> AMDPEFETGEVVDCHLSDMLQQLHSVNASKPSERGLVRQEEAEDPACIPIFWVSKWVDYSDKYGLGYQLCDNSVGVLFNDSTRLILYNDGDSLQYIERDGTESYLTVSSHPNSLMKKITLLKYFRNYMSEHLLKAGANITPREGDELARLPYLRTWFRTRSAIILHLSNGSVQINFF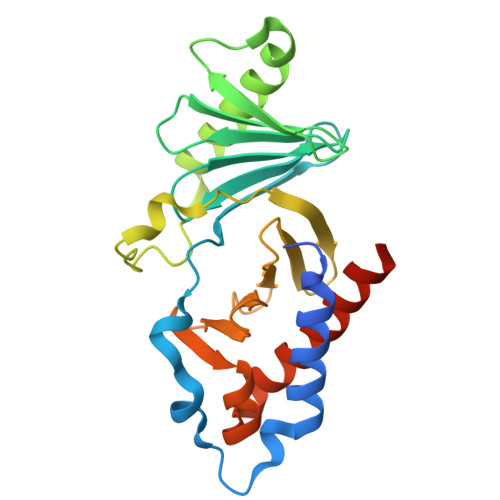QDHTKLILCPLMAAVTYIDEKRDFRTYRLSLLEEYGCCKELASRLRYARTMVDKLLSSRSASNRLKAS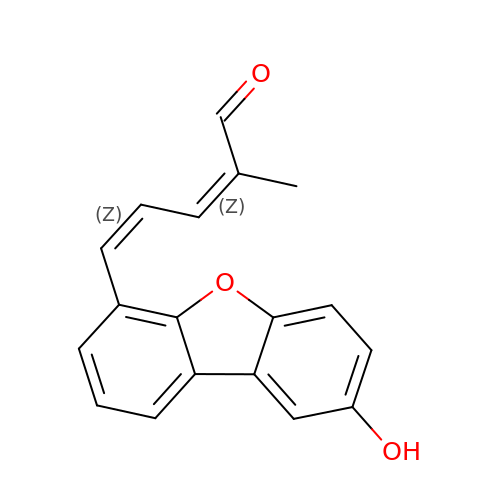(2~{Z},4~{Z})-2-methyl-5-(8-oxidanyldibenzofuran-4-yl)penta-2,4-dienal | C18 H14 O3 | FWMQKXGLKVAFDC-FYOBGJLRSA-N>GSHMPNLCVSATFNPPVITMLGSALREETVKLLEQRIPTGVSTSSSPSKDPVKFLFYPNPDHWRMELSQHFCDDLHKSAVFLTIIEGLEGE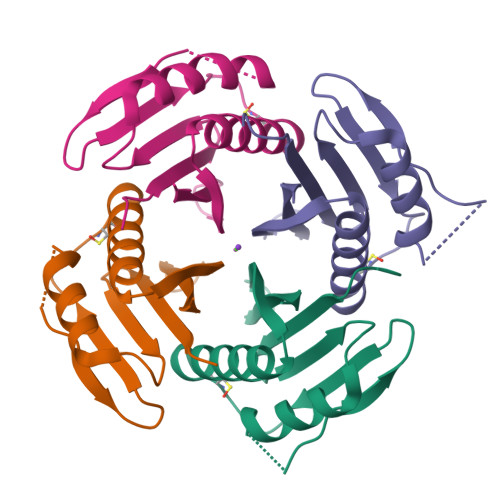GWNLRASNSIRDSESGKDTTKLFFARRN[4x]> YNLDVRGARSFSPPRAGRHFGYRVLQVGNGVIVGAPGEGNSTGSLYQCQSGTGHCLPVTLRGSNYTSKYLGMTLATDPTDGSILACDPGLSRTCDQNTYLSGLCYLFRQNLQGPMLQGRPGFQECIKGNVDLVFLFDGSMSLQPDEFQKILDFMKDVMKKLSNTSYQFAAVQFSTSYKTEFDFSDYVKWKDPDALLKHVKHMLLLTNTFGAINYVATEVFREELGARPDATKVLIIITDGEATDSGNIDAAKDIIRYIIGIGKHFQTKESQETLHKFASKPASEFVKILDTFEKLKDLFTELQKKIYVIEGTSKQDLTSFNMELSSSGISADLSRGHAVVGAVGAKDWAGGFLDLKADLQDDTFIGNEPLTPEVRAGYLGYTVTWLPSRQKTSLLASGAPRYQHMGRVLLFQEPQGGGHWSQVQTIHGTQIGSYFGGELCGVDVDQDGETELLLIGAPLFYGEQRGGRVFIYQRRQLGFEEVSELQGDPGYPLGRFGEAITALTDINGDGLVDVAVGAPLEEQGAVYIFNGRHGGLSPQPSQRIEGTQVLSGIQWFGRSIHGVKDLEGDGLADVAVGAESQMIVLSSRPVVDMVTLMSFSPAEIPVHEVECSYSTSNKMKEGVNITICFQIKSLIPQFQGRLVARLTYTLQLDGHRTRRRGLFPGGRHELRRNIAVTTSMSCTDFSFHFPVCVQDLISPIRVSLNFSLWEEEGTPRDQRAQGKDIPPILRPSLHSETWEIPFEKNPAALQTLFQGPLGAQGEKELQALEKENAQLEWELQALEKELAQHHHHHHA;> QECTKFKVSSCRECIESGPGCTWCQKLNFTGPGDPDSIRCDTRPQLLMRGCAADDIMDPTSLAETQEDHNGGQKQLSPQKVTLYLRPGQAAAFNVTFRRAKGYPIDLYYLMDLSYSMLDDLRNVKKL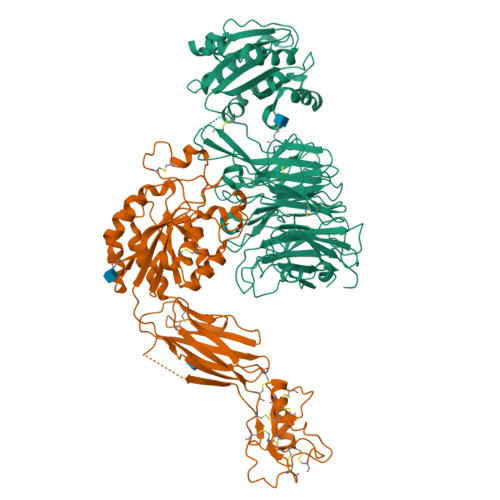GGDLLRALNEITESGRIGFGSFVDKTVLPFVNTHPDKLRNPCPNKEKECQPPFAFRHVLKLTNNSNQFQTEVGKQLISGNLDAPEGGLDAMMQVAACPEEIGWRKVTRLLVFATDDGFHFAGDGKLGAILTPNDGRCHLEDNLYKRSNEFDYPSVGQLAHKLAENNIQPIFAVTSRMVKTYEKLTEIIPKSAVGELSEDSSNVVQLIKNAYNKLSSRVFLDHNALPDTLKVTYDSFCSNGVTHRNQPRGDCDGVQINVPITFQVKVTATECIQEQSFVIRALGFTDIVTVQVLPQCECRCRDQSRDRSLCHGKGFLECGICRCDTGYIGKNCEPAALQTLFQGPLGAQGKKKLQALKKKNAQLKWKLQALKKKLAQHHHHHHA>[2x]MVMAKYDVLTIGNAIVDIIARCDDSFLEENGIIKGAMNLINADRAELLYSRMGPAVEASGGSAGNTAAGVASLGGRAAYFGKVADDQLGEIFTHDIRAQGVHFQTKPLDGHPPTARSMIFVTEDGERSMNTYLGACVELGPEDVEDDVVAQSKVTYFEGYLWDPPRAKDAIREAARIAHAHGRETAMTLSDSFCVHRYRSEFLELMRSGTVDIVFANRQEALALYETEDFDRALELLARDCKLAAVTLSE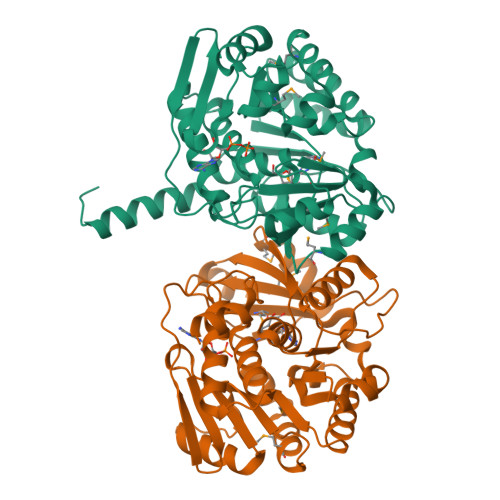EGSVVVRGAERVRVGASVLEQVVDTTGAGDLYAAGFLFGYTSGRSLEECSKLGNLAAGIVIGQIGPRPLVSLATAARQAALVAENLYFQSHHHHHHWSHPQFEK>[2x]GPHMMAAKVLLVEDDRALREALSDTLLLGG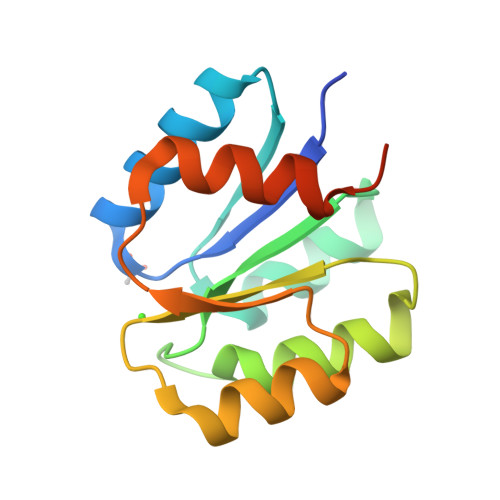HEFVAVDSAEAALPVLAREAFSLVISDVNMPGMDGHQLLGLIRTRYPHLPVLLMTAYGAVDRAVEAMRQGAADYLVKPFEARALLDLVARHALGQLPGSEEDGP>SNAMITMTEVKGKTANESRVFKTSRVFPTDLNDHNTLFGGKILSEMDMVASISASRHSRKECVTASMDWVDFLHPVRSSDCVSYESFVIWTGRTSMEVFVKVVSEYLISGEKRIAATSFVTFVALSKENNPVPVPRVIPDTE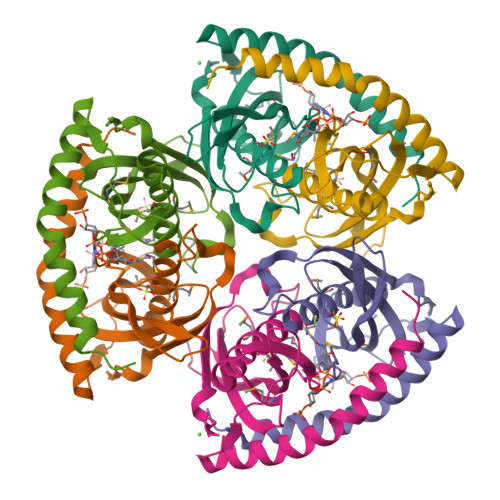EEKESHRIAVLRAEQRHIRKAESKKVATLLTF[3x]>[4x]MRVLVLLACLAAASNAGSQYETYQWDEDYDQEPDDDYQTGFPFRQNVDYGVPFHQYTLGCVSECFCPTNFPSSMYCDNRKLKTIPNIPMHIQQLYLQFNEIEAVTANSFINATHLKEINLSHNKIKSQKIDYGVFAKLPNLLQLHLEHNNLEEFPFPLPKSLERL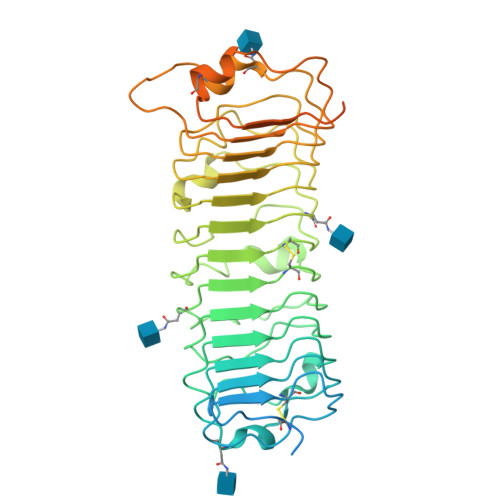LLGYNEISKLQTNAMDGLVNLTMLDLCYNYLHDSLLKDKIFAKMEKLMQLNLCSNRLESMPPGLPSSLMYLSLENNSISSIPEKYFDKLPKLHTLRMSHNKLQDIPYNIFNLPNIVELSVGHNKLKQAFYIPRNLEHLYLQNNEIEKMNLTVMCPSIDPLHYHHLTYIRVDQNKLKEPISSYIFFCFPHIHTIYYGEQRSTNGQTIQLKTQVFRRFPDDDDESEDHDDPDNAHESPEQEGAEGHFDLHYYENQEAAADYKDDDDK>[2x]AMNYFVGNSLGVNLTGIEKAIINRLNLFKEMGRPAQCVFLSWNRYLYRNAQNYITSSDYINMYDFFQEATYLERNEPFDWLSYWTDECHYTLKHVENSHDFRIYDQERFLMYAHFQDPKYRILDYVNHFDSQRRKVKRDFYDVRGFLSCSRILVDKQQTLCEFFYNPEGDTKLEKYFSYKDGKPEVQKIIVYYANKQYFFNNETELGAFFIKQLYQHGDLFFSDRNVYTAPIFNLTPESIPVVAVLHSTHIKNIDALDSSPFKNVYKAMFENLSRYRAIIVSTEQQKLDVEKRINHTIPVVNIPVGYSETIDTPVQTLDQRSVKLISVARYSPEKQLHQQIELIKRLVSYVPKIELHMYGFGSESKKLNELIQKYGLENHVYLRGFLSNLDQEYSDAYLSLITSNMEGFSLALLESLAHGVPVISYDIKYGPNELITSDFNGYLITKNDEDALFDKVKYVIDHPEVQQRLSKGSLAKAQQYSKASLIKQWDQFVRLILEHHHHHH;>[2x]DSDSDSDSD

Two glycosyltransferases (GTases), SdgB and SdgA, are responsible for the glycosylation of S. aureus SDR proteins such as ClfA and ClfB. SdgB first appends N-acetyl­glucosamine (GlcNAc) moieties onto serine residues (O-glycosylation) within the SDR domain using uridine diphos­phate N-acetylglucosamine (UDP-GlcNAc) as a donor substrate. The subsequent addition of GlcNAc to the glycoproteins is catalyzed by the second enzyme, SdgA, yielding glycosylated SDR proteins in which each SD repeat is decorated with GlcNAc disaccharide moieties. The glycosylation of SDR proteins mediated by SdgA and SdgB protects SDR proteins from degradation by host proteases, thereby circumventing innate immune attack.

Despite the biological significance of these two glycosyltransferases involved in pathogenicity and avoidance of the host innate immune response, their structures and the molecular basis of their activity have not been investigated. This study reports the crystal structures of SdgB and SdgA from S. aureus as well as multiple structures of SdgB in complex with its substrates (for example UDP, N-acetylglucosamine or SDR peptides), products (glycosylated SDR peptides) or phosphate ions. Interestingly, SdgB undergoes a conformational change from an open to closed complex upon substrate binding. In addition to the dimerization role, the inserted domain was found to serve as a binding platform for the SD repeats before and after glycosylation. A long positive tract along the inserted domain stabilizes the binding of the glycosylated SD repeats to SdgB by offsetting the negative charge clustered in the tandem SD repeats. SdgB and SdgA share the way that they recognize monoglycosylated SD repeats as a product and a substrate, respectively, but SdgA is likely to preferentially bind a longer SDR substrate than a shorter one.> MPHEYEKDGAKIYVQSFATIRAEADLARFTPEEEVVVVRMIHAAGMVGLENHVRFAPGMAIAARAALEAGAPILCDARMVSEGITRARLPAKNEVICTLQDPRVPALAQEMGNTRSAAALELWRPKLEGAVVAIGNAPTALFHLLNM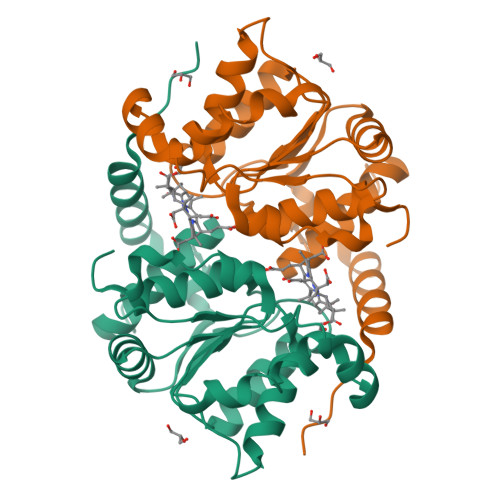LEDPACPRPAAIIGCPVGFIGAAESKAALAVANPVPWVIVEGRLGGSAITVAAVNALACRKE2-(4-fluorophenyl)-1-{4-[(isoquinolin-5-yl)sulfonyl]piperazin-1-yl}ethan-1-one | C21 H20 F N3 O3 S | 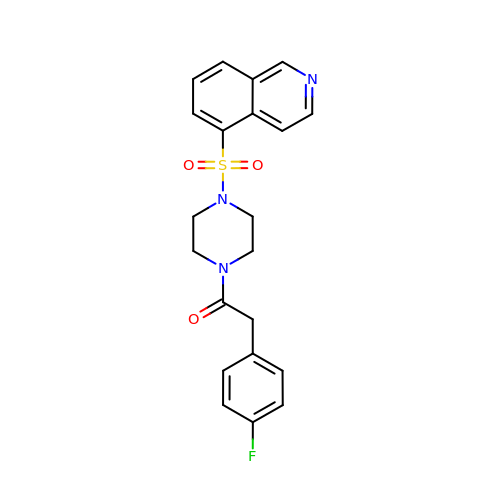MVUOZWVYTYXUCV-UHFFFAOYSA-N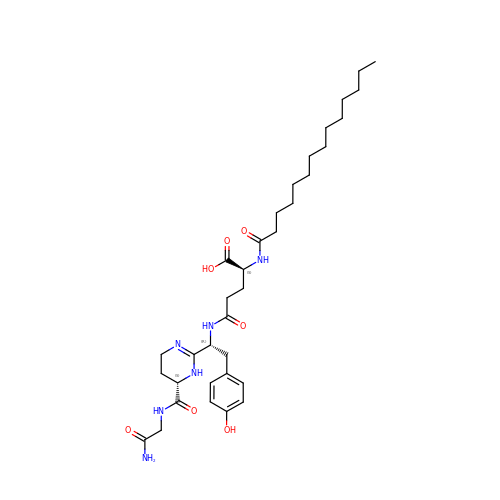N-[(1R)-1-{(6S)-6-[(2-amino-2-oxoethyl)carbamoyl]-1,4,5,6-tetrahydropyrimidin-2-yl}-2-(4-hydroxyphenyl)ethyl]-N~2~-tetradecanoyl-L-glutamine | C34 H54 N6 O7 | DGAYEIHJKULBKL-HZFUHODCSA-N>[8x]AFAKIEEGKLVIHMPAAVAVTSPQADSAPAQRFSLPQGC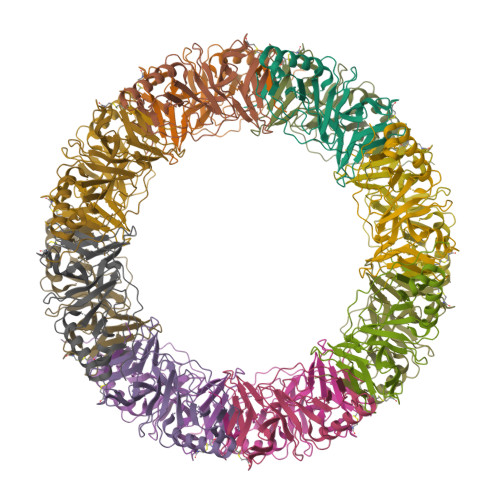HFRTFWRDEANGGSLFIPAGDALRCGEDGWLQGSGAVTLQQGGQTLSPTLWFLQGYPLAQVNGGDRALTVVSANAQRLILGGNPQAPGSFLLLTFEPQLHAWAFNGEAIVEMPRVDAADETKIKQRVQQAQTAWQPLLSAPAPLTFKLVEKLAADRVDPASGSYLSVNGATHLEGSEFKLVDHHHHHH>CCATTA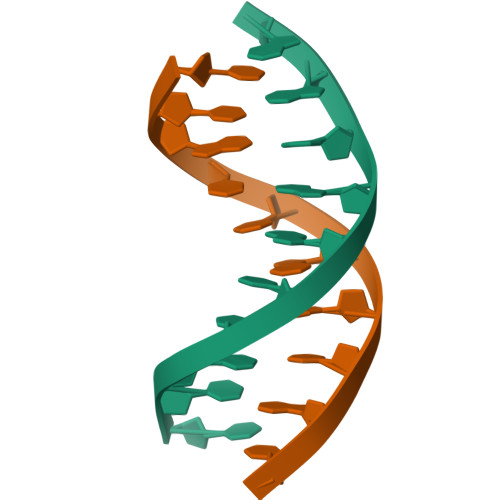ATGG[2x]> MIDKSAFVHPTAIVEEGASIGANAHIGPFCIVGPHVEIGEGTVLKSHVVVNGHTKIGRDNEIYQFASIGEVNQDLKYAGEPTRVEIGDRNRIRESVTIHRGTV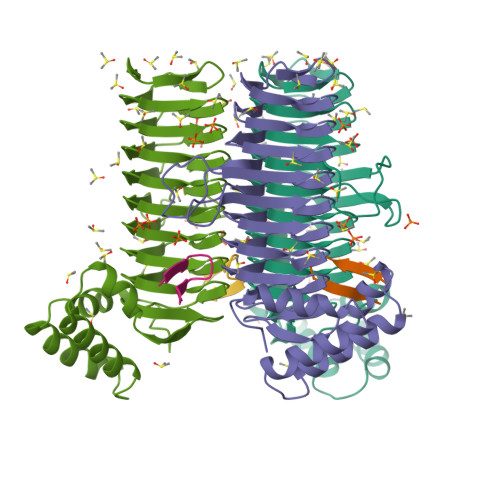QGGGLTKVGSDNLLMINAHIAHDCTVGNRCILANNATLAGHVSVDDFAIIGGMTAVHQFCIIGAHVMVGGCSGVAQDVPPYVIAQGNHATPFGVNIEGLKRRGFSREAITAIRNAYKLIYRSGKTLDEVKPEIAELAETYPEVKAFTDFFARSTRGLIR;> SSGWMLDPIAGKWSR>MGLFDRIKRVVSSNLNDLVNKAEDPEKMLEQAILEMQEDLVQLRQGVAQAIAAQKRSEKQYNDAQNEINKWQRNAQLALQKGDENLARQALERKKTYTDTSAALKASLDTQSTQVETLKRNLIQLESKISEAKTKKEMLKARITTAKAQEQLQGMVRGMNTSSAMSAFERMEEKVLMQESRAQALGELAGADLETQFAQLEGGSDVDDELAALKAQMLPPATPVTQAQLPPQQETTPAKSNEVVDAELDSLRKQLDQL[78x]

Proteins that perform these functions include Vipp1/IM30 in photosynthetic plastids, PspA in bacteria, and ESCRT-III in eukaryotes. Here, using a combination of evolutionary and structural analyses, we show that these protein families are homologous and share a common ancient evolutionary origin that likely predates the last universal common ancestor. This homology is evident in cryo-electron microscopy structures of Vipp1 rings from the cyanobacterium Nostoc punctiforme presented over a range of symmetries. Rings have an inner lumen that is able to bind and deform membranes.

Reconstructions were also generated for the other six symmetries and complete ring models built. Rungs are maximally constricted at the top and bottom with internal lumen diameters of 14 nm and 15.7 nm, and widest at the ring equator between rungs 3 and 4 with an internal diameter of 17.5 nm. This unique asymmetric curvature is a feature of all Vipp1C11–C17 ring symmetries. The analysis of different ring symmetries, ranging from C11–C17, provides us with a view of the structural flexibility that enables Vipp1, PspA, and ESCRT-III family members to perform their functions. Furthermore, as each ring comprises between 5–7 rungs stacked together to build a dome-shaped architecture, these asymmetric structures provide us with a glimpse of the structural features that enable filament tilt in the context of an ESCRT-III-like polymer. Based on the Vipp1C11–C17 models, where helix α5C is positioned at the tip of the spike, α6 helices likely coat the ring outside surface and do not contribute directly to polymer formation. Consistent with this, Interfaces 1 and 3 linking the top two rungs were poorly resolved in Vipp1C11–C17 rings, indicating a weak interaction once the limiting geometry is reached. When membrane was modeled into the Vipp1C11–C17 structures as a 4-nm bilayer, sequential constriction was observed with the membrane lumen reaching ∼3 nm within Vipp1C11.(2S)-2-[3-(3-chlorophenyl)phenyl]-2-methyl-5,6-dihydro-1,3-oxazin-4-amine 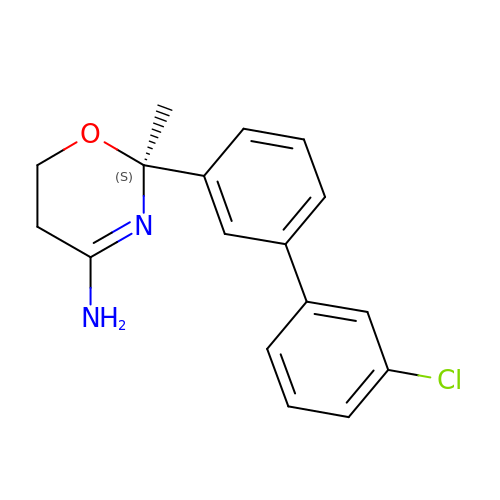| C17 H17 Cl N2 O | DAWFJSNCVYTRMO-KRWDZBQOSA-N>[3x]HHHHHHSSGLVPRGSPESLALPNDFEWGFATAAYQIEGAVKEGGRGPSIWDTYCHLEPSRTNGANGDVACDHYHRYDEDFDLLTKYGAKAYRFSLSWSRIIPLGGRLDPVNEEGIEFYSKLIDALLRRGITPWVTLYHWDLPQALHDRYGGWLNVEEVQLDFERYARLCFERFGDRVQNWITINEPWIQAIYGYATGSNAPGRSSINKHSTEGDTATEPWLAGKAQIMSHARAVAVYSRDFRPSQKGQIGISLNGDYYEPWDSNEPRDKEAAERRMEFHIGWFANPIFLKKDYPESMKKQLGERLPALTPADFAILNAGETDFYGMNYYTSQYARHLDGPVPETDYLGAIHEHQENKDGSPVGEESGLAWLRSCPDMFRKHLARVYGLYGKPIYITENGCPCPGEENMTCEEAVNDPFRIRYFDSHLDSISKAITQDGVVVKGYFAWALLDNLEWSDGYGPRFGVTF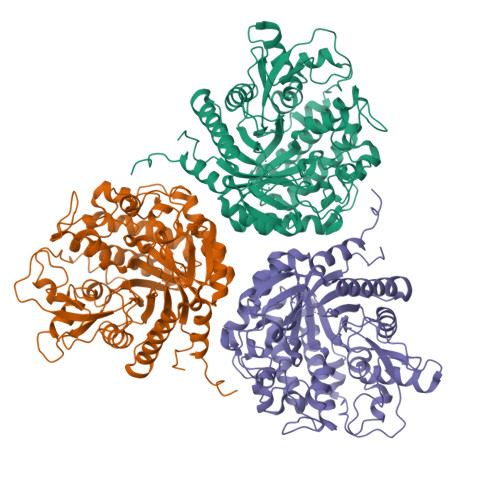TDYTTLKRTPKKSALVLKDMFAARQIPEELAHLADLKFLEHHHHHH> PPPP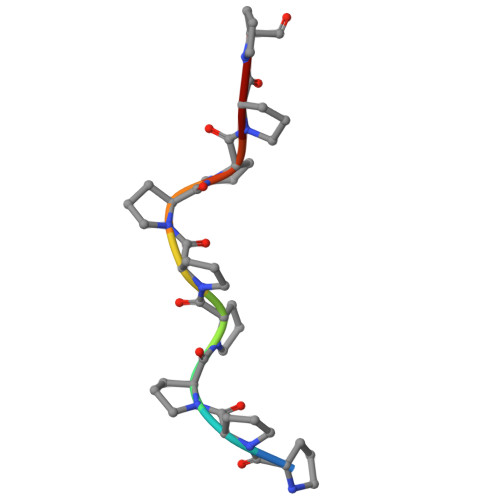PPPPP>MMDKFRMIFQFLQSNQESFMNGICGIMALASAQMYSAFDFNCPCLPGYNAAYSAGILLAPPLVLFLLGLVMNNNVSMLAEEWKRPPGRRAKDPAVLRYMFCSMAQRALIAPVVWVAVTLLDGKCFLCAFCTAVPVSALGNGSLAPGLPAPELARLLARVPCPEIYDGDWLLAREVAVRYLRCISQALGWSFVLLTTLLAFVVRSVRPCFTQAAFLKSKYWSHYIDIERKLFDETCTEHAKAFAKVCIQQFFEAMNHDLELGHTNGTLATAPASAAAPTTPDGAEEEREKLRGITDQGTMNRLLGSAWSHPQFEK[8x]

Calcium homeostasis modulator 1 (CALHM1) is a voltage-dependent channel involved in neuromodulation and gustatory signaling. CALHM1 is the recently identified member of a large-pore channel that permeates ions, including Ca2+, Na+, K+, and Cl−, and small molecules, such as ATP, in a voltage-dependent manner. Furthermore, the ATP efflux through the CALHM1 channel in type II gustatory cells and the subsequent purinergic signaling has been shown to facilitate the perception of sweet, bitter, and umami taste sensations. Our studies here showed that the human and chicken CALHM1s have a conserved structural fold, oligomeric assembly pattern, and a phospholipid-filled hydrophobic pocket for controlling channel functions.

To compare structures and assembly patterns of mammalian and non-mammalian CALHM1 channels, we determined the cryo-EM structure of human CALHM1, as well as that of chicken CALHM1 prepared using an identical protocol. Our single-particle cryoEM resulted in the octameric chCALHM1Δct and hCALHM1Δct structures, resolved at the overall resolutions of 3.36 and 3.76 Å, respectively. The structures revealed that the chCALHM1Δct and hCALHM1Δct protomers have a similar protein fold and octameric assembly pattern, where the C-terminal helix (CTH) and TMD4-CTH linker are the major determinants for controlling the oligomeric state. As is the case for non-mammalian CALHM1s, the most extensive inter-subunit interactions form between the TMD2 and TMD4 and between the CTHs in hCALHM1. Our hCALHM1Δct structure allows mapping of key residues for functions and human mutations, Pro86Leu and Arg154His, implicated as risks of Alzheimer’s disease. In our hCALHM1Δct structure, the cryo-EM density was resolved up to Pro85 but not Pro86. Arg154 is surrounded by residues, Arg158 and Gly139, from the neighboring subunit in the hCALHM1Δct. Additionally, Asp121, which has been reported to modulate calcium sensitivity and ion permeability, is located on TMD3 and at the inter-subunit interface with TMD4 from the neighboring subunit to contribute to the structural integrity of the oligomer. Inspection of the hCALHM1Δct and chCALHM1Δct structures reveals a hydrophobic pocket ~15 Å in length (parallel to the TMDs) and 10 Å wide, located between TMD3 and TMD4 of one subunit and TMD2 of the neighboring subunit. In both hCALHM1Δct and chCALHM1Δct, we observe phospholipid-like density nestled into this pocket, which appears to fortify the local architecture by interacting with the hydrophobic residues in the pocket.>GHMPNIPPPFTAPYAPDDAEIAARLLPASHLSPPQEARIHRTATRLIEAIRKRDDRLGGVEDMLREFALSTKEGLALMVLAEALLRVPDARTADQFIEDKLGEGDFIHHETKSTAFLVNASAWALGLSARVIQPGETPDGTIGRLVKRLGAPAVRTATRQAMRLMGNHFVLGETIEQALERGKPRSGQKTRYSFDMLGEGARTAADARRYFDAYASAIETIGKAAGNHALPDRPGISVKLSALHPRFEAISRARVMVELVPQLLDLAQRAKAHDLNFTVDAEEADRLELSLDVIAATLADPSLKGWDGFGLAIQAYQKRASAVIDYVDALARAHDRKLMVRLVKGAYWDTEIKRAQERGLDGYPVFTRKAMTDLNYVACASKLLALRPRIFPQFATHNALTVATVLEMAEGSSGFEFQRLHGMGEALYEQLAKDHADIAYRTYAPVGSHRDLLAYLVRRLLENGANSSFVAQAADYRVPVPALLQRPADAIVRPQAAAHPRIPLPCDLFAPERRNSRGVEFGARTALDQLLTDVKAETGDLKPIADATPDQAHAAVAAARAGFAGWSRTPAGIRAAALEQAAHLLESRSAHFIALLQREGGKTLDDALSELREAADFCRYYAAQGRKLFGSETAMPGPTGESNALTMRGRGVFVAISPWNFPLAIFLGQVTAALMAGNSVVAKPAEQTPRIAREAVALLHEAGIPKSALYLVTGDGRIGAALTAHPDIAGVVFTGSTEVARSINRALAAKDGPIVPLIAETGGINAMIADATALPEQVADDVVTSAFRSAGQRASALRLLFVQEDVADRMIEMVAGAARELKIGDPSDVATHVGPVIDVEAKQRLDAHIARMKTEARLHFAGPAPEGCFVAPHIFELTEAGQLTEEVFGPILHVVRYRPENLERVLRAIERTGYGLTLGVHSRIDDSIEAIIDRVQVGNIYVNRNMIGAVVGVQPFGGNGLSGTGPKAGGPHYLARFATEQTVTINTAAAGGNAALLAGEE[2x]

Proline utilization A (PutA) proteins are bifunctional enzymes that catalyze the oxidation of l-proline to l-glutamate. PutAs contain two spatially separated active sites that catalyze the two reactions of proline catabolism. The proline dehydrogenase (PRODH) active site catalyzes the oxidation of proline to Δ1-pyrroline-5-carboxylate (P5C) with concomitant reduction of the flavin adenine dinucleotide (FAD) cofactor. The intermediate P5C is in equilibrium with its hydrolysis product, l-glutamate-γ-semialdehyde (GSAL). The latter species is the substrate for the GSAL dehydrogenase (GSALDH) active site of PutA, which catalyzes the nicotinamide adenine dinucleotide (NAD+)-dependent oxidation of GSAL to glutamate.

The BjPutA C792A variant was used for X-ray crystallography. Cys792 is the catalytic cysteine of the GSALDH active site, and C792A is devoid of GSALDH activity, but has wild-type PRODH activity. Soaking the crystals in 2 M proline bleached the yellow color, consistent with reduction of the FAD cofactor. X-ray diffraction data were collected on a flash-cooled crystal, and the structure was determined at a 2.15 Å resolution. The asymmetric unit of the C2 crystal form contains a BjPutA dimer. The dimer is a domain-swapped assembly in which the oligomerization domain of one protomer engages the GSALDH module of the other protomer. Although the degree of bending is lower in BjPutA C792A, the direction of bending is the same as in other reduced PutAs. These results confirm the FAD in the BjPutA C792A structure is reduced. Nine proline molecules were modeled into 5 sites. Three of the sites are functionally significant: (1) the GSAL binding site of the GSALDH module; (2) the NAD+ site; and (3) the substrate-channeling tunnel. Accordingly, proline in the GSAL site has the highest occupancy (1.0) and lowest B-factor of all the sites.>[4x]A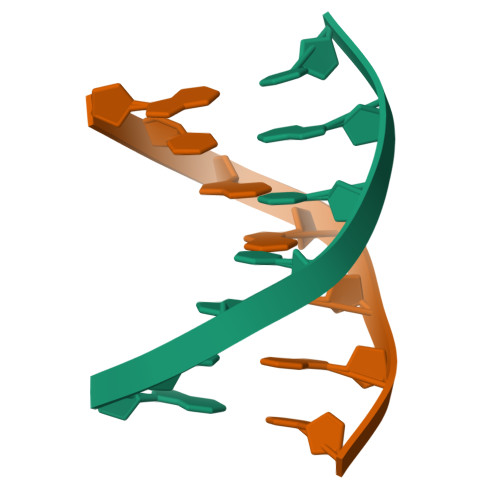CGCCGT;>ACGICGT[4x]> APDTSVSNKQNFSTDVIYQIFTDRFSDGNPANNPTGAAFDGTCTNLRLYCGGDWQGIINKINDGYLTGMGVTAIWISQPVENIYSIINYSGVNNTAYHGYWARDFKKTNPAYGTIADFQNLIAAAHAKNIKVIIDFAPNHTSPASSDQPSFAENGRLYDNGTLLGGYTNDTQNLFHHNGGTDFSTTENGIYKNLFDLADLNHNNSTVDVYLKDAIKMWLDLGIDGIRMDAVKHMPFGWQKSFMAAVNNYKPVFTFGEWFLGVNEVSPENHKFANESGMSLLDFRFAQKVRQVFRDNTDNMYGLKAMLEGSAADYA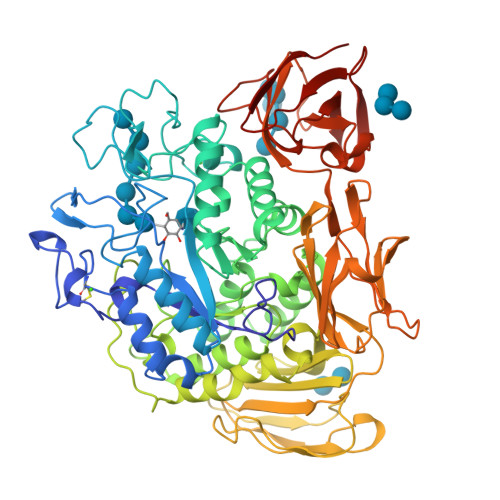QVDDQVTFIDNHDMERFHASNANRRKLEQALAFTLTSRGVPAIYYGTEQYMSGGTDPDNRARIPSFSTSTTAYQVIQKLAPLRKCNPAIAYGSTQERWINNDVLIYERKFGSNVAVVAVNRNLNAPASISGLVTSLPQGSYNDVLGGLLNGNTLSVGSGGAASNFTLAAGGTAVWQYTAATATPTIGHVGPMMAKPGVTITIDGRGFGSSKGTVYFGTTAVSGADITSWEDTQIKVKIPAVAGGNYNIKVANAAGTASNVYDNFEVLSGDQVSVRFVVNNATTALGQNVYLTGSVSELGNWDPAKAIGPMYNQVVYQYPNWYYDVSVPAGKTIEFKFLKKQGSTVTWEGGSNHTFTAPSSGTATINVNWQP> HGHSSSDPVYPCGICTNEVND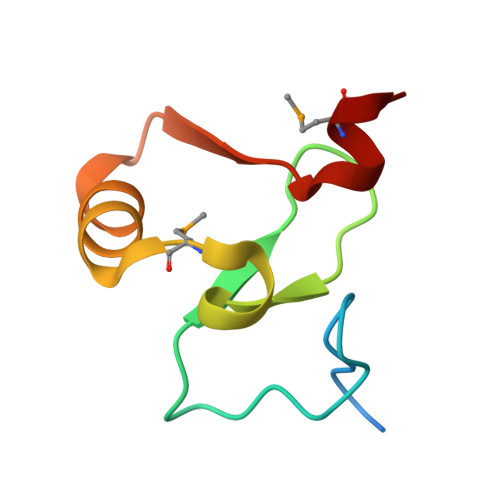DQDAILCEASCQKWFHRICTGMTETAYGLLTAEASAVWGCDTCMAD>SELSFNYPNFQSVEDITFQGGASPRNETLQLTPTDSNGIPIRQRAGHAVYSQPFQLRDTSFYTTFTFVIRTTSNSPADGFAIFIAPPDFPVKRYGGYLGLFEPNTATNTSANKVVAVEFDTWVNTEWKEPRYRHIGIDVNSIVSVRVTRWQDKDVFSRSIATAHVGYDGISKILTAFVTYPDGGNYVLSHVVDLAEIFPGDVRIGFSGATGQYETQYIHSWSFSSTSTNLLRDGARHHHHHH[2x];>XSSVG[2x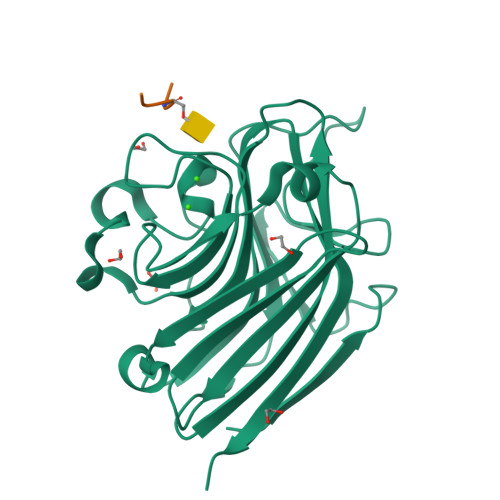]> MDAKARNCLLQHREALEKDIKTSYIMDHMISNGVLSVIEEEKVKSQATQYQRAAALIKMILNKDNCAYISFYNALLHEGYKDLAALLQSGLPLVSSSSGKDTDGGITSFVRTVLCEGGVPQRPVIFVTRKKLVHAIQQKLWKLNGEPGWVTIYGMAGCGKSVLAAEAVRDHSLLEGCFSGGVHWVSIGKQDKSGLLMKLQNLCMRLDQEESFSQRLPLNIEEAKDRLRVLMLRKHPRSLLILDDVWDPWVLKAFDNQCQILLTTRDKSVTDSVMGPKHVVPVESGLGREKGLEILSLFVNMKKEDLPAEAHSIIKECKGSPLVVSLIGALLRDFPNRWAYYLRQLQNKQFKRIRKSSSYDYEALDEAMSISVEMLREDIKDYYTDLSILQKDVKVPTKVLCVLWDLETEEVEDILQEFVNKSLLFCNRNGKSFCYYLHDLQVDFLTEKNRSQLQDLHRKMVTQFQRYYQPHTLSPDQEDCMYWYNFLAYHMASANMHKELCALMFSLDWIKAKTELVGPAHLIHEFVAYRHILDEKDCAVCENFQEFLSLNGHLLGRQPFPNIVQLGLCEPETSEVYRQAKLQAKQEGDTGRLYLEWINKKTIKNLSRLVVRPHTDAVYHACFSQDGQRIASCGADKTLQVFKAETGEKLLDIKAHEDEVLCCAFSSDDSYIATCSADKKVKIWDSATGKLVHTYDEHSEQVNCCHFTNKSNHLLLATGSNDFFLKLWDLNQKECRNTMFGHTNSVNHCRFSPDDELLASCSADGTLRLWDVRSANERKSINVKRFFLSSEDPPED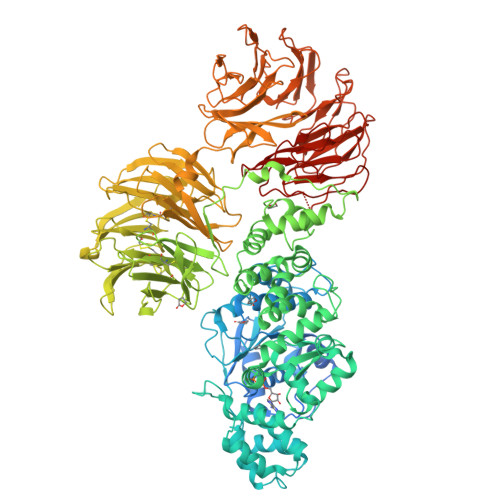VEVIVKCCSWSADGDKIIVAAKNKVLLFDIHTSGLLAEIHTGHHSTIQYCDFSPYDHLAVIALSQYCVELWNIDSRLKVADCRGHLSWVHGVMFSPDGSSFLTASDDQTIRVWETKKVCKNSAIVLKQEIDVVFQENETMVLAVDNIRGLQLIAGKTGQIDYLPEAQVSCCCLSPHLEYVAFGDEDGAIKIIELPNNRVFSSGVGHKKAVRHIQFTADGKTLISSSEDSVIQVWNWQTGDYVFLQAHQETVKDFRLLQDSRLLSWSFDGTVKVWNVITGRIERDFTCHQGTVLSCAISSDATKFSSTSADKTAKIWSFDLLSPLHELKGHNGCVRCSAFSLDGILLATGDDNGEIRIWNVSDGQLLHSCAPISVEEGTATHGGWVTDVCFSPDSKTLVSAGGYLKWWNVATGDSSQTFYTNGTNLKKIHVSPDFRTYVTVDNLGILYILQVLE>AQPFAHLTINAASIPSGSHKVTLSSWYHDRGWAKISNMTLSNGKLRVNQDGFYYLYANICFRHHETSGSVPTDY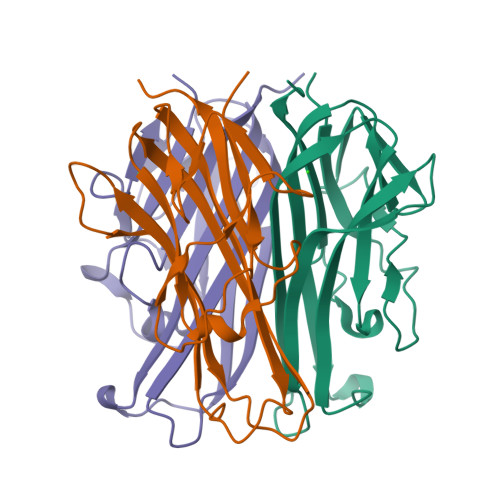LQLMVYVVKTSIKIPSSHNLMKGGSTKNWSGNSEFHFYSINVGGFFKLRAGEEISIQVSNPSLLDPDQDATYFGAFKVQDID[3x]Kivd, a thiamine diphosphate (ThDP)-dependent 2-keto acid decarboxylase, belongs to the pyruvate decarboxylase family and exhibits broad substrate specificity. Kivd, the key enzyme in this pathway, catalyzes the conversion of 2-ketoisovalerate into isobutyraldehyde, which has been identified as a bottleneck in IB production. The enzyme demonstrates the highest affinity for 2-ketoisovalerate, an intermediate in the biosynthesis of the branched-chain amino acid valine. KivdS286T is a key enzyme in the 2-keto acid pathway, catalyzing the conversion of 2-ketoisovalerate (KIV) and 2-ketoisocaproate (KIC) to isobutyaldehyde and isovaleraldehyde, respectively, in Synechocystis sp. PCC 6803 (Synechocystis).

The 2.8 Å X-ray crystal structure of KivdS286T reveals a tetrameric assembly composed of four polypeptide chains. The tetrameric structure is consistent with the results obtained from gel filtration chromatography, confirming that the crystal structure of KivdS286T represents the biologically active form of the protein. Due to low electron density in the X-ray crystallographic data, several disordered regions were not modeled. These regions include residues 181–187 in chains A and B, and residues 180–195 in chains C and D. In addition, residues from 456 to 477 and from 529 to 548 in the C-terminal region of chains C and D were not included in the model. Each KivdS286T monomer consists of three distinct domains. The N-terminal PYR domain binds the pyrimidine ring of ThDP, the central R domain lacks bound cofactors, and the C-terminal PP domain interacts with the diphosphate group of ThDP. The enzyme’s active site is located at the interface between the PP and PYR domains of adjacent monomers. The ThDP cofactor, crucial for the decarboxylation reaction, is anchored within the active site through interactions with the conserved GDGX25-30NN motif, which coordinates with the diphosphate tail and an Mg2+ ion. Based on the tetrameric crystal structure of KivdS286T, one dimer contains the essential cofactors ThDP and Mg2+, which are required for the catalytic function of KivdS286T. Interestingly, the adjacent dimer lacks these cofactors.

>[4x]MYTVGDYLLDRLHELGIEEIFGVPGDYNLQFLDQIISHKDMKWVGNANELNASYMADGYARTKKAAAFLTTFGVGELSAVNGLAGSYAENLPVVEIVGSPTSKVQNEGKFVHHTLADGDFKHFMKMHEPVTAARTLLTAENATVEIDRVLSALLKERKPVYINLPVDVAAAKAEKPSLPLKKENSTSNTSDQEILNKIQESLKNAKKPIVITGHEIISFGLEKTVTQFISKTKLPITTLNFGKSSVDEALPSFLGIYNGTLSEPNLKEFVESADFILMLGVKLTDTSTGAFTHHLNENKMISLNIDEGKIFNERIQNFDFESLISSLLDLSEIEYKGKYIDKKQEDFVPSNALLSQDRLWQAVENLTQSNETIVAEQGTSFFGASSIFLKSKSHFIGQPLWGSIGYTFPAALGSQIADKESRHLLFIGDGSLQLTVQELGLAIREKINPICFIINNDGYTVEREIHGPNQSYNDIPMWNYSKLPESFGATEDRVVSKIVRTENEFVSVMKEAQADPNRMYWIELILAKEGAPKVLKKMGKLFAEQNKS>[2x]NSCASKEEVVPSPEEGQCSQESVKQSFVTRFTECSLSPEVGEGPYFIEEDIIRSNIV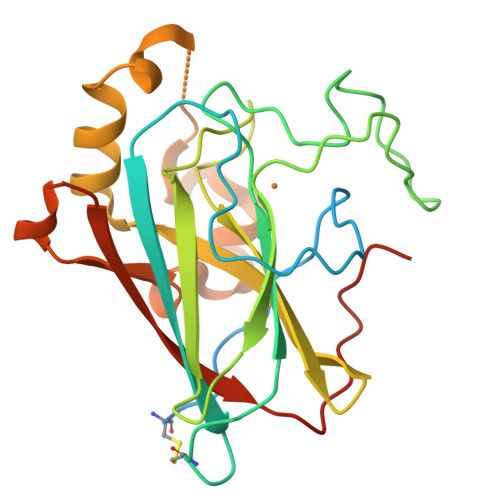EDRIGIRLNVTLNLVDFNTCKPIKGAKVYIWQPDYSGIYSGFMDKPRVKREKMYPKDPRRFLRGTQVTNENGTVTFETLFPGHYPGRTPHIHYRIHANGNVAHIGQIFFDESTSQVIQSKSPYNQVHSRRMKNEEDGEFTYFNGKKSIINIDPQSLSGDSLEGILNLAINPLHRSNLMWAAGENLYFQ> MQDAITSVINSSDVQGKYLDASAIQKLKAYFATGELRVRAATTISANAANIVKEAVAKSLLYSDVTRPGGNMYTT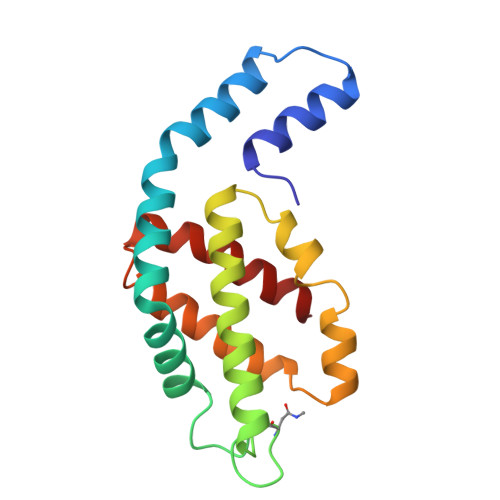RRYAACIRDLDYYLRYATYAMLAGDPSILDERVLNGLKETYNSLGVPIGATVQAIQAMKEVTAGLVGGGAGKEMGIYFDYICSGLS>[4x]MGHHHHHHHHHHSSGHIEGRHMMATNLRGVMAALLTPFDQQQALDKASLRRLVQFNIQQGIDGLYVGGSTGEAFVQSLSEREQVLEIVAEEAKGKIKLIAHVGCVSTAESQQLAASAKRYGFDAVSAVTPFYYPFSFEEHCDHYRAIIDSADGLPMVVYNIPALSGVKLTLDQINTLVT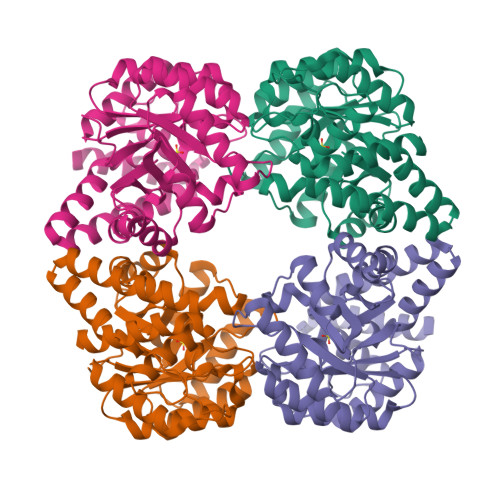LPGVGALKQTSGDLYQMEQIRREHPDLVLYNGYDEIFASGLLAGADGGIGSTYNIMGWRYQGIVKALKEGDIQTAQKLQTECNKVIDLLIKTGVFRGLKTVLHYMDVVSVPLCRKPFGPVDEKYLPELKALAQQLMQERG> MRGSHHHHHHGSAVSAKIEIYTWSTCPFCMRALALLKRKGVEFQEYCIDGDNEAREAMAARANGKRSLPQIFIDDQHIGGCDDIYILDGAGKLDPLLHS

In the case of the glutaredoxin that is the focus of this study, glutaredoxin A from the cyanobacterium Synechocystis sp. PCC 6803 serves as the preferred electron donor for the 2-electron reduction of arsenate to arsenite, catalyzed by arsenate reductase. As part of the thioredoxin superfamily, glutaredoxin A shares the characteristic thioredoxin fold. The structure of the wild-type protein is comprised of the major protein secondary structure elements: four α-helical segments, and four mixed parallel: anti-parallel β-strands that form a single β-pleated sheet. Our random mutagenesis approach has yielded four new crystal structures of glutaredoxin A, one for each of the following variants: R27L, A75I, A79S, and P84R.

Due to the location of Ala75, one might have predicted that changes in structure and function observed for the A75I and the A79S variants would be subtle. These replacements are located at the extreme C-terminus of the protein in α-helix 4, and both are exposed to the outside surface of the helix. Neither is involved in crystal packing interactions nor core packing interactions, and therefore, these positions are predicted to be highly tolerant of modification. Since ammonium sulfate is used in the crystallization medium of these glutaredoxin A crystals, there are two sulfate anions coordinated to the wild-type and to the mutated glutaredoxin A structures. Interestingly, the A75I mutation does not coordinate sulfate ions in its crystal structure. In the wild-type structure, sulfate #2 is 10.6 Å from the Cα atom of Ile75, while sulfate #1 is 35.2 Å distant. The large distance between the site of the mutation and the ligand binding site discounts any direct effect on sulfate binding. As there is no sulfate anion bound to the N-terminus, the His-tag of A75I is considerably more disordered that the other glutaredoxin structures that do coordinate sulfate. The same residues in the A75I structure without a coordinated sulfate anion show an average temperature factor of 32.6 Å2. While the elevated temperature factors can be explained by the lack of sulfate coordination, the rationale for the lack of this anion in this mutation is still unknown.>[6x]ATPHINAEMGDFADVVLMPGDPLRAKYIAETFLEDAREVNNVRGMLGFTGTYKGRKISVMGHGMGIPSCSI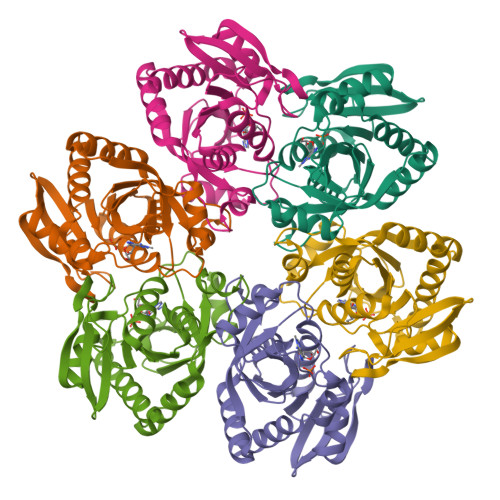YTKELITDFGVKKIIRVGSCGAVLPHVKLRDVVIGMGACTDSKVNRIRFKDHDFAAIADFDMVRNAVDAAKALGIDARVGNLFSADLFYSPDGEMFDVMEKYGILGVEMEAAGIYGVAAEFGAKALTICTVSDHIRTHEQTTAAERQTTFNDMIKIALESVLLGDK>GSHMASEELQKDLEEVKVLLEKATRKRVRDA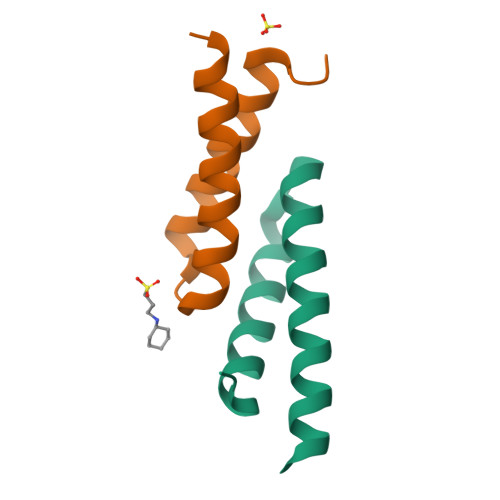LTAEKSKIETEIKNKMQQK[3x]> MIVIFVDFDYFFAQVEEVLNPQYKGKPLVVCVYSGRTKTSGAVATANYEARKLGVKAGMPIIKAMQIAPSAIYVPMRKPIYEAFSNRIMNLLNKHADKIEVASIDEAYLDVTNKVEGNFENGIELARKIKQEILEKEKITVTVGVAPNKILAKIIADKSKPNGLGVIRPTEVQDFLNELDIDEIPGIGSVLARRLNELGIQKLRDILSKNYNELEKITGKAKALYLLKLAQDEYN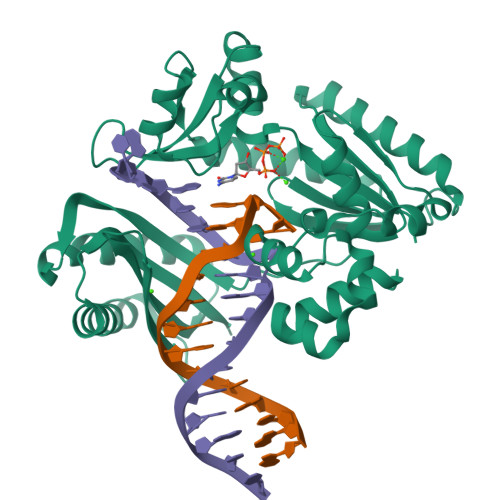EPIRTRVRKSIGRIVTMKRNSRNLEEIKPYLFRAIEESYYKLDKRIPKAIHVVAVTEDLDIVSRGRTFPHGISKETAYSESVKLLQKILEEDERKIRRIGVRFSKFIEAIGLDKFFDTGGHHHHHH>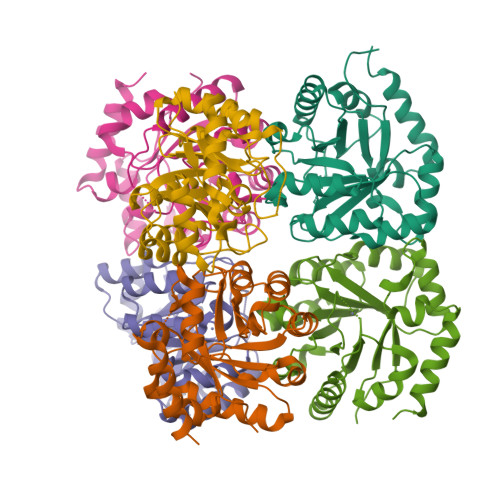[6x]MAHHHHHHMQPFAIAPSILSADFARLGEDVDKVLAAGADIVHFDVMDNHYVPNLTIGPMVCSALRKYGVSAPIDVHLMVSPVDRIIGDFIEAGATYITFHPEASQHIDRSLQLIRDGGCKAGLVFNPATPLEVLKYVMDKVDMVLLMSVNPGFGGQKFIPGTLDKLREARALIDASGREIRLEIDGGVNVKNIREIAAAGADTFVAGSAIFNAPDYAEVIRAMHAELAQAHQ> MGIDINTKIFNSVAEVFQKAQGSYAGHRKHIAVLKKIQSKAVEQGYEDAFNFWFDKLVTKILPLKKNEIIGDRIVKLVAAFIASLERELILAKKQNYKLTNDEEGIFSRFVDQFIRHVLRGVESPDKNVRFRVLQLLAVIMDNIGEIDESLFNLLILSLNKRIYDREPTVRIQAVFCLTKFQDEEQTEHLTELSDNEENFEATRTLVASIQNDPSAEVRRAAMLNLINDNNTRPYILERARDVNIVNRRLVYSRILKSMGRKCFDDIEPHIFDQLIEWGLEDRELSVRNACKRLIAHDWLNALDGDLIELLEKLDVSRSSVCVKAIEALFQSRPDILSKIKFPESIWKDFTVEIAFLFRAIYLYCLDNNITEMLEENFPEASKLSEHLNHYILLRYHHNDISNDSQSHFDYNTLEFIIEQLSIAAERYDYSDEVGRRSMLTVVRNMLALTTLSEPLIKIGIRVMKSLSINEKDFVTMAIEIINDIRDDDIEKQESESDIINNLPPEKEASSATIVLCLTRSSYMLELVNTPLTENILIASLMDTLITPAVRNTAPNIRELGVKNLGLCCLLDVKLAIDNMYILGMCVSKGNASLKYIALQVIVDIFSVHGNTVVDGEGKVDSISLHKIFYKVLKNNGLPECQVIAAEGLCKLFLADVFTDDDLFETLVLSYFSPINSSNEALVQAFAFCIPVYCFSHPAHQQRMSRTAADILLRLCVLWDDLQSSVIPEVDREAMLKPNIIFQQLL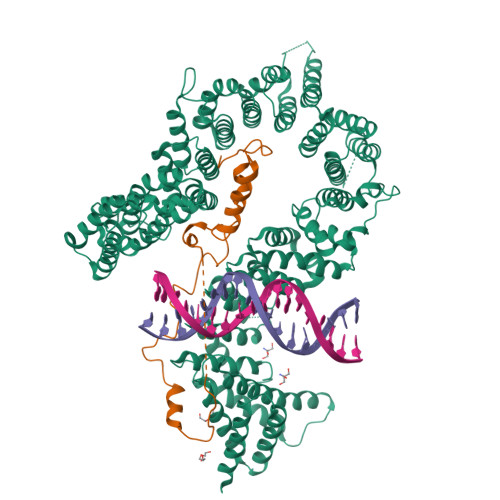FWTDPRNLVNQTGSTKKDTVQLTFLIDVLKIYAQIEKKEIKKMIITNINAIFLSSEQDYSTLKELLEYSDDIAENDNLDNVSKNALDKLRNNLNSLIEEINERSETQTKDENNTANDQYSSILGN;> GPLGHMSIFEKDLMAYFDENLNRNWRGREHWKVRNFKKANLVNKESDLLEETRTTIGDTTDKNTTDDKSMDTKKKHKQKKVLEIDFFKTDDSFEDKVFASKGRTKIDMPIKNRKNDTHYLLPDDFHFSTDRITRLFIKPGQKMSLFSHRKHT> MPRLIKERVPTPERSVGERVRDFGEVNLGYSWELALREAERCLQCPVEYAPCIKGCPVHINIPGFIKALRENRDNPSKAVREALRIIWRDNTLPAITGRVCPQEEQCEGACVVGKVGDPINIGKLERFVADYAREHGIDDELLLEEIKGIKRNGKKVAIIGAGPAGLTCAADLAKMGYEVTIYEALHQPGGVLTYGIPEFRLPKEILRKELKKLSLLGVEIKTDHIVGKTITIQELLQEYDAVFIGTGAGTPKLPNIPGINLNGIYSANEFLTRINLMKAYKFPEYDTPIVVGKKVVVIGAGNTAMDAARSALRLGAEVTIAYRRGREDMTARIEEVKHAEEEGVKFMFFVNPVEFIGDENGNVKAVKFEKMKPLEERDSRGKRKIVGTGEYITVEADTVIIAIGQTPNKVLWRATPELKV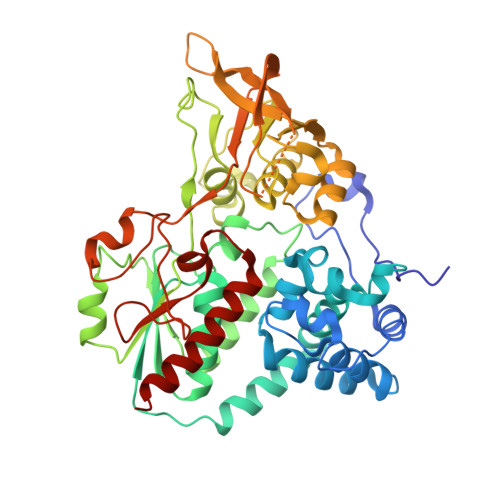DEWGRIVVDENLMTSIPGVFAGGDAIRGEATVILAMGDGRKAAKAIHQYLSKKGN>MKKNAKQIVHELYNDISISKDPKYSDILEVLQKVYLKLEKQKYELDPSPLINRLVNYLYFTAYTNK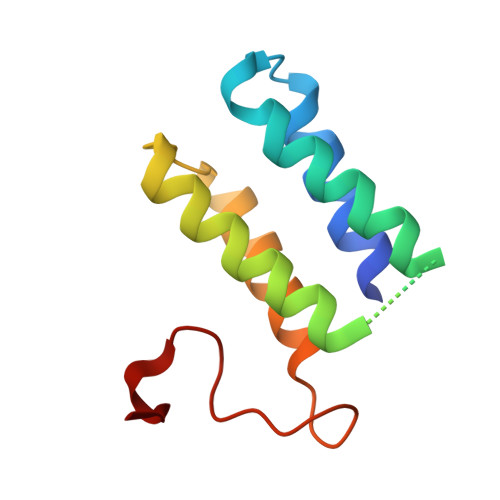IRFTEYQEELIRNLSEIGRTAGINGLYRADYGDKSQF[3x]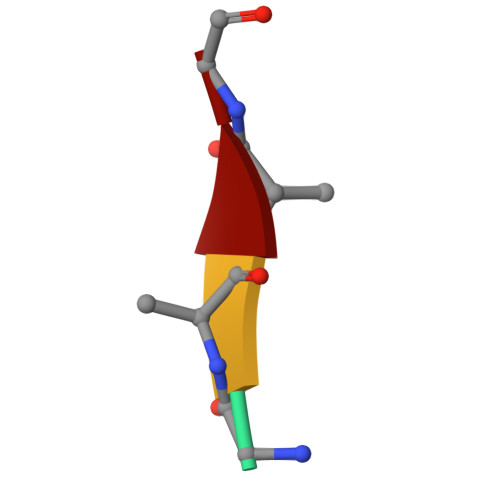> GAAG> MDAKTTILE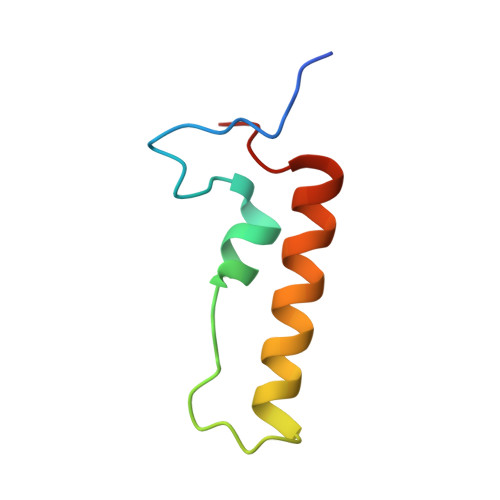VLKKEGKPMSAGQIAEKSGLERKEVDKAMKSLKEEELIVSPKRCYWTPKV>[2x]PRVVFIDEQSGEYAVDAQD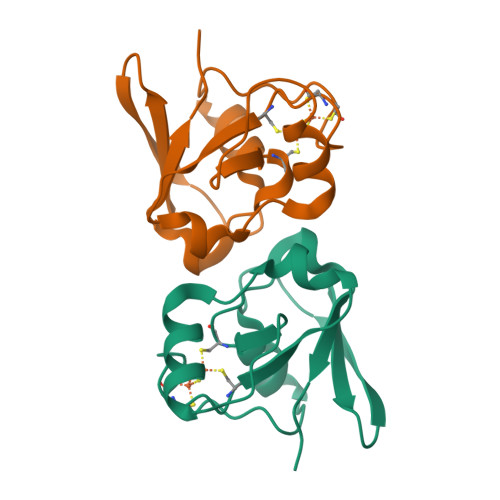GQSLMEVATQNGVPGIVAECGGSSVCATCRIEIEDAWVEIVGEANPDENDLLQSTGEPMTAGTRLSCQVFIDPSMDGLIVRVPLPA>[4x]DEEVQEAVERAEELREEAEELIKKARKTGDPELLRKALEALKEAVRAVKEAIKRNPDNEEAVKTAVRLARELLKVAEELKERAEKTGDPRLLLLAAEAIAWAIEAVFLAAKASENTEGALEAARAAVKLAEVAKRIAKLLQRDAKKEGDPELLKLALRALELAVRAVELAIKENPDNEEAVETAKRLAEELRKVAELLEERAKETGDPELQELAKRA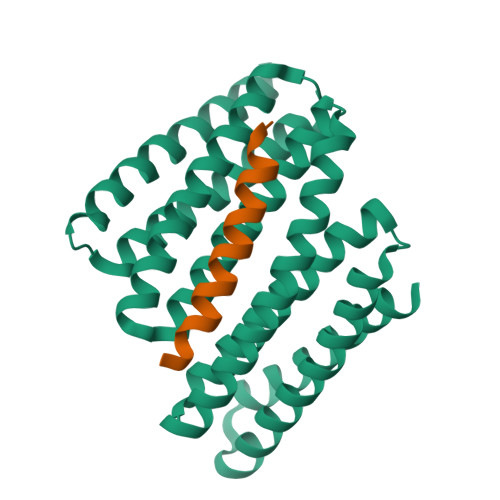KEVADRARELAKKSNPNNSEEQEAARLLELAVEDLKLVLDALEKRR> SNAASEGTSGIIASFYDSLVTQAAGEDVRSSNDDEHFLTWGVFQEIVPGFSWIRTVFRPSERPEGRERLAVAQRELRRVLFRAVDLSAIKNVMDFGCGHGSDLIILGEQNEHLKLDGYTISGKQAEVCKQRVRTRGLQNRIRIFQRDSAKDDFPGMYDLV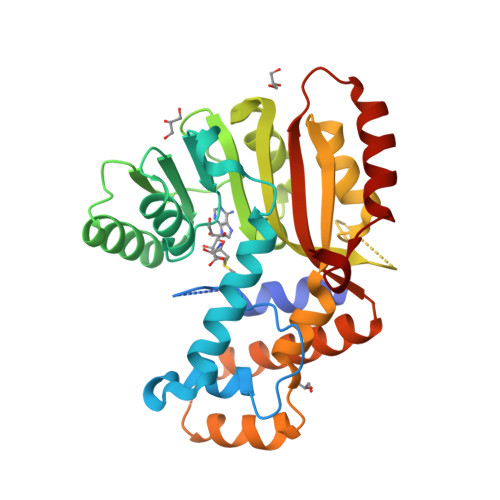LGFEVAGLIPDKDALFSNIDRHLTNGGLLIMADFVANTLSPIEVQETSTFSSTREQWNKLFSSNHLRLVDAVDVSNEVANCLHNPDYAAQFEALCKELKLDEVTQRSFGSYENVYKALRGGLISYVLFHVQKDRFSRSDELFHLNAKQFEQLTPYAEFA>[4x]GSFSAADVYVPDEWEVAREKITMSRELGQGSFGMVYEGVAKGVVKDEPETRVAIKTVNEAASMRERIEFLNEASVMKEFNCHHVVRLLGVVSQGQPTLVIMELMTRGDLKSYLRSLRPEMENNPVLAPPSLSKMIQMAGEIADGMAYLNANKFVHRDLAARNCMVAEDFTVKIGDFGMTRDIYETDYYRKGGKGLLPVRWMSPESLKDGVFTTYSDVWS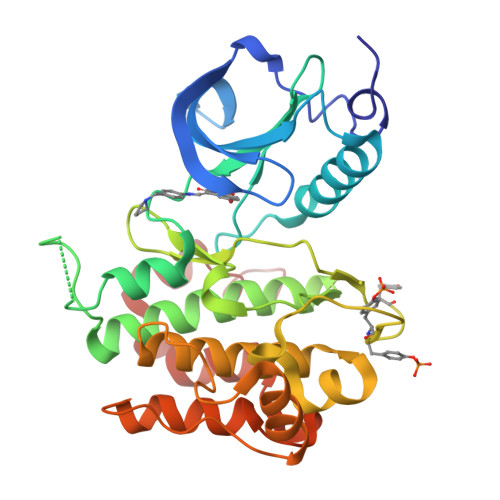FGVVLWEIATLAEQPYQGLSNEQVLRFVMEGGLLDKPDNCPDMLFELMRMCWQYNPKMRPSFLEIISSIKEEMEPGFREVSFYYSEENK> AHHHHHHMQGSVTEFLKPRLVDIEQVSSTHAKVTLEPLERGFGHTLGNALRRILLSSMPGCAVTEVEIDGVLHEYSTKEGVQEDILEILLNLKGLAVRVQGKDEVILTLNKSGIGPVTAADITHDGDVEIVKPQHVICHLTDENASISMRIKVQRGRGY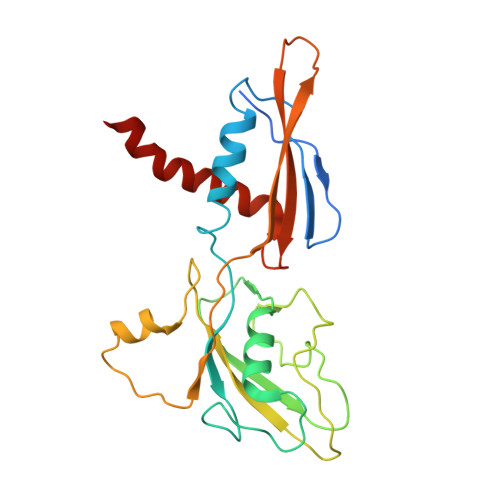VPASTRIHSEEDERPIGRLLVDACYSPVERIAYNVEAARVEQRTDLDKLVIEMETNGTIDPEEAIRRAATILAEQLEAFVDLR L-GLUCARIC ACID | C6 H10 O8 | 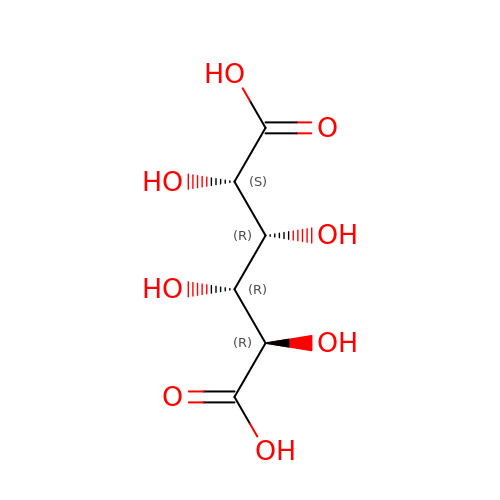DSLZVSRJTYRBFB-AJSXGEPRSA-N>[2x]S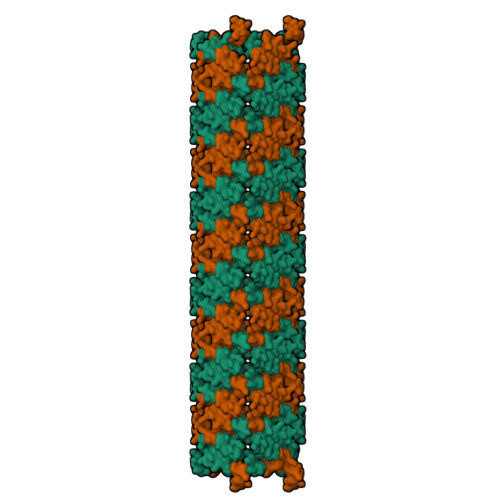KRIVQRIKDFLR> GMKTRDKIIQASLELFNEHGERT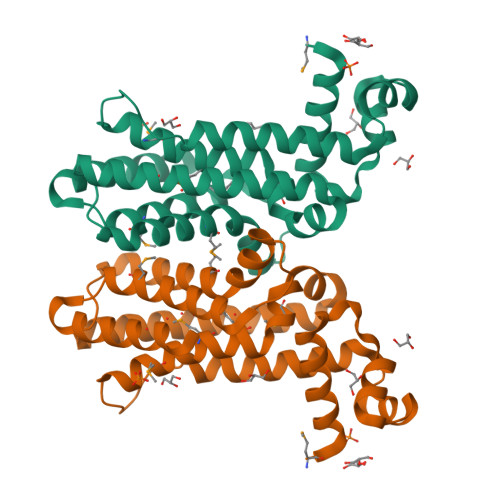ITTNHIAAHLDISPGNLYYHFRNKEDIIRCIFDQYEQHLLLGFKPYADQKVDLELLMSYFDAMFYTMWQFRFMYANLADILARDDTLKARYLKVQQAVLEQSIAVLNQLKKDGILQIEDERIADLADTIKMIIGFWISYKLTQSSIATISKASLYEGLLRVLMIFKAYSTPDSLANFDRLEQHFRSQSN>[6x]MKMVVAVIRPEKLECVKKALEERGFVGMTVTEVKGRGEQKGIRLQFRGREVEVDLLQKTKVEVVVSDDAVDEVVEAIVSSARTGKFGDGRIFVIPVEKSVKIRTGDEEVAAAHHHHHH

PII proteins are key sensors for the metabolic nitrogen status. Af-GlnK3 shares the canonical fold of PII proteins, consisting of a four-stranded, antiparallel beta sheet and two connecting alpha helices. It forms a tightly packed trimer with approximate dimensions of 30×54 Å. GlnK proteins, when activated, are sequestered to the cytoplasmic membrane where they bind directly to their corresponding Amt proteins, physically blocking ammonium uptake by inserting the T-loops deeply into the transporters' substrate channels.

MgATP and MgADP bound to the protein in a highly conserved nucleotide-binding pocket, a cleft located at the interface of two monomers where the ligands are in direct contact with the B-, C- and the T-loop. As under good nutritional conditions the ATP/ADP ratio in the cell is presumed to be high, the ATP-bound state of Af-GlnK3 should represent the common physiological situation, signaling a state of sufficient metabolic energy. Even in crystallization trials with high concentrations of magnesium salts, no Mg2+ ions could be unambiguously identified in the binding pocket. Structural variations in the conformation of the three phosphate moieties of the ATP ligand were observed within the asymmetric unit, and the T-loops were still disordered. The bulky γ-phosphate moiety cannot be accommodated without breaking both the salt bridge between Glu 38 and Lys 101 and the hydrogen bond between Glu 39 and Lys 58. In consequence, the base of the T-loop loses its fixation points and the entire region becomes disordered. Whether this state of the protein is competent to associate with the Amt protein remains to be elucidated.> GPHVKSGLQIKKNAIIDDYKVTSQVLGLGINGKVLQIFNKRTQEKFALKMLQDCPKARREVELHWRASQCPHIVRIVDVYENLYAGRKCLLIVMECLDGG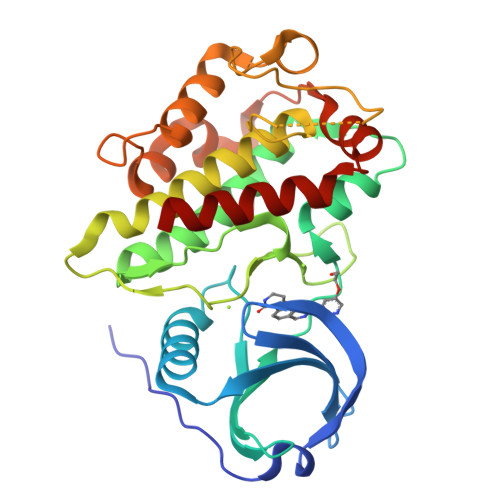ELFSRIQDRGDQAFTEREASEIMKSIGEAIQYLHSINIAHRDVKPENLLYTSKRPNAILKLTDFGFAKETTGEKYDKSCDMWSLGVIMYILLCGYPPFYSNHGLAISPGMKTRIRMGQYEFPNPEWSEVSEEVKMLIRNLLKTEPTQRMTITEFMNHPWIMQSTKVPQTPLHTSRVLKEDKERWEDVKEEMTSALATMR Neurofibromin 2 belongs to the FERM (band 4.1, ezrin, radixin, moesin) gene family characterized by an N-terminal FERM domain that binds to the plasma membrane, a central α-helical domain, and a C-terminal tail domain that binds to the cortical actin cytoskeleton. Neurofibromin 2 is a unique tumor suppressor protein that inhibits cell growth both from plasma membrane and in the nucleus upon cell confluency. The neurofibromin 2 head–tail interaction is critical for controlling the tumor-suppressive function of neurofibromin 215,16, which seems also to be regulated by phosphorylation.

Here we report the crystal structure of the neurofibromin 2 N-terminal domain in complex with PIP2, which reveals a large conformational change upon lipid binding. The crystal structure contains two polypeptide chains, two polyethylene glycols, two phosphates, and two PIP2 molecules in the asymmetric unit. In both polypeptide chains, the PIP2 inositol head group is sandwiched between Trp-60 and Arg-309, the 5′ inositol phosphate interacts with the backbone of Arg-310 and the 1-phosphate group is in hydrogen-bonding distance to Arg-309. The oxygen atoms of the diacylglycerol interact with the hydroxyl group of Thr-59. While the lipid-bound FERM domain part of the structure (residues 21–312) resembles the apo FERM structure, the α-helix of the helical domain αH undergoes a large structural change and adopts a distinct conformation. In the apo structure, a short loop (residues 312–315) allows αH to interact with the F1 FERM subdomain (specifically by electrostatic interactions of Arg-57 with Asp-314). Upon PIP2 binding, the acyl group stacks with the side chain of Arg-57 at this interface and severs the FERM and αH interaction further by exposing its 5′ phosphate group into the solvent. This causes the loop (residues 312–315) that keeps αH interacting with F1 in the apo structure, to become helical, and thereby extending the last F3 α-helix (residues 290–312) to form one continuous long α-helix (residues 290–339) instead in the lipid-bound structure by a ~60° relative rotation. Importantly, in our lipid-bound structure, the F3 subdomain is in the conformer seen in the apo structure in the space that is occupied by the tail domain in the head/tail structure.

>[2x]MAGAIASRMSFSSLKRKQPKTFTVRIVTMDAEMEFNCEMKWKGKDLFDLVCRTLGLRETWFFGLQYTIKDTVAWLKMDKKVLDHDVSKEEPVTFHFLAKFYPENAEEELVQEITQHLFFLQVKKQILDEKIYCPPEASVLLASYAVQAKYGDYDPSVHKRGFLAQEELLPKRVINLYQMTPEMWEERITAWYAEHRGRARDEAEMEYLKIAQDLEMYGVNYFAIRNKKGTELLLGVDALGLHIYDPENRLTPKISFPWNEIRNISYSDKEFTIKPLDKKIDVFKFNSSKLRVNKLILQLCIENHDLFMRRRKADSLEVQQMKAQAREEKARKQMERQRL> MAISFDNALGIHQHTVGVRERNAEVISTNIAQANTPGYKARGLDFAKELQAATSGASIGLSRT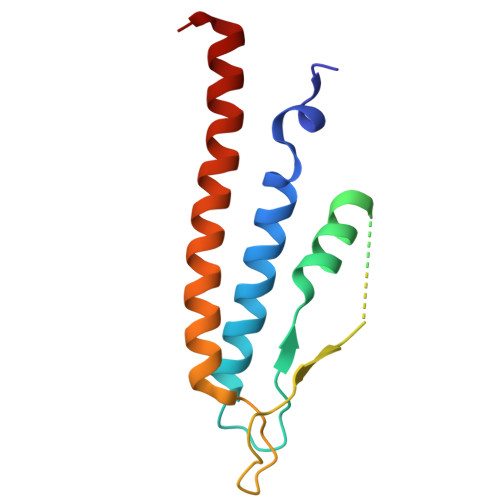DGRHIPATTTLVGDKLYRLPTQPDTGDGNTVDLDLERNLFMQNQIRHQASLDFLGSKFKNLTKAIKGE> SGKGKGKRTHFNQFAYDGNTY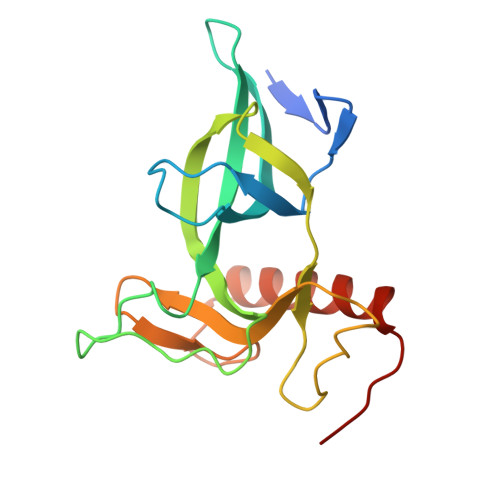DLEVPVLLVPEDKSQKPYVAIIKDITQTKDGSMMILGQWFYRPEEAEKRGGGNWQSSDTRELFYSFHRDEVPAESVMHRCVVYFVPAHKQLPKRKNNPGFIVRKVYDTVEKKLWKLTDKDYEDSKQREIDVLVKKTMNVLGDLPDLES> GPHMPEKLEAILIPDQGYHQVGPADLCTDMFVLSVTVAFATKLEQLVPSTMKLSAEGSEFFFYYSLLGNDITSEPFHNLLSPDFEPERASVRIRSSKQILKAFLSQQPSLQIHLCCGNHSLGSTDVSLSALAGISTDLDNKAA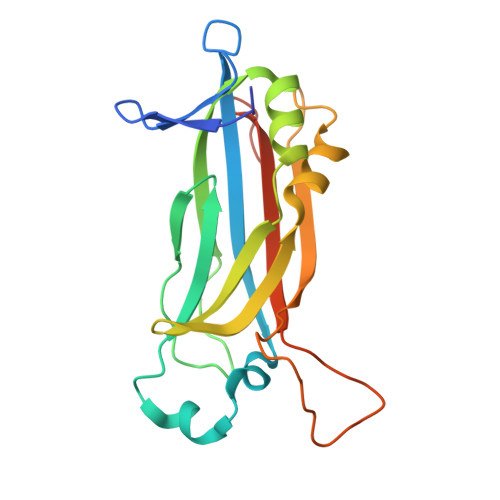TVEGAFILQPPKRVKQTLPALPTDLQPTLGVAVTLRREEVALQQSVGNKE3-(4-PHENYLAMINO-PHENYLAMINO)-2-(1H-TETRAZOL-5-YL)-ACRYLONITRILE 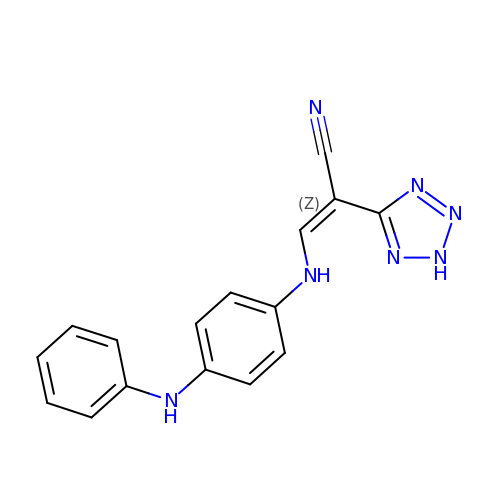| C16 H13 N7 | FLPLCJJGNZGOAW-QXMHVHEDSA-N>GDIVSEKKPATEVDPTHFEKRFLKRIRDLGEGHFGKVELCRYDPEGDNTGEQVAVKSLKPESGGNHIADLKKEIEILRNLYHENIVKYKGICTEDGGNGIKLIMEFLPSGSLKEYLPKNKNKINLKQQLKYAVQICKGMDYLGSRQYVHRDLAARNVLVESEHQVKIGD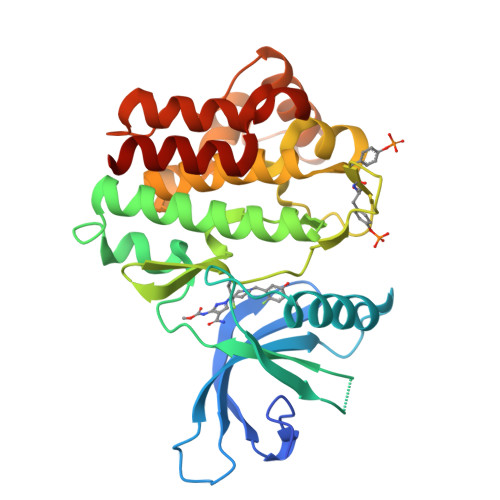FGLTKAIETDKEYYTVKDDRDSPVFWYAPECLMQSKFYIASDVWSFGVTLHELLTYCDSDSSPMALFLKMIGPTHGQMTVTRLVNTLKEGKRLPCPPNCPDEVYQLMRKCWEFQPSNRTSFQNLIEGFEALLK[2x]>[4x]AMGSATISRRGILVIRHGERVDQVFGKSWLQQCTTADGKYYRPDLNFPRSLPRRSN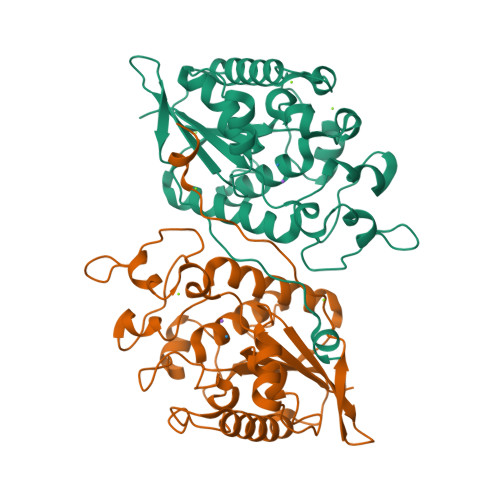GIKDFENDPPLSSCGIFQARLAGEALLDSGVRVTAVFASPALRCVQTAKHILEELKLEKKLKIRVEPGIFEWMKWEASKATLTFLTLEELKEANFNVDLDYRPALPRCSLMPAESYDQYVERCAVSMGQIINTCPQDMGITLIVSHSSALDSCTRPLLGLPPRECGDFAQLVRKIPSLGMCFCEENREDGKWDLVNPPVKTLTHGANSVFNWRNWIS> AVINHDAVPVWPQPEPADATQALAVRFKPQLDVVNGCQPYPAVDPQGNTSGGLKPSGSQAAACRDMSKAQVYSRSGTYNGYYDIMYSWYMPKDSPSIGIGHRHDWENVVVWLDNAASANIVALSASAHSGYKKSFPADKSYLDGITAKISYKSTWPLDHELGFTTSAGKQQPLIQWEQMTQAARDALESTD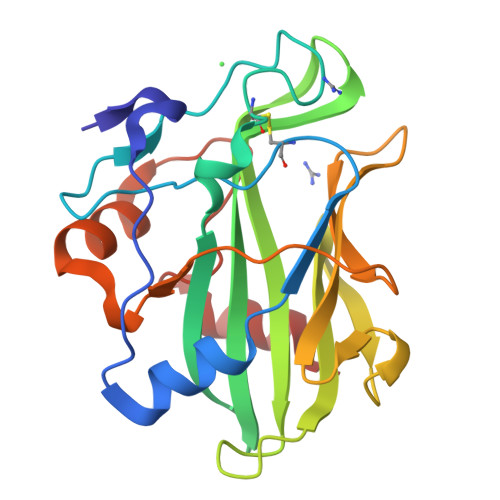FGNANVPFKSNFQDKLVKAFFQ>[2x]SQVRTYPNGLIVEELSMGKPNGKRADPGKTVSVRYIGKLQKNGKIFDSNIGKSPFKFRLGIGSVIKGWDVGVNGMR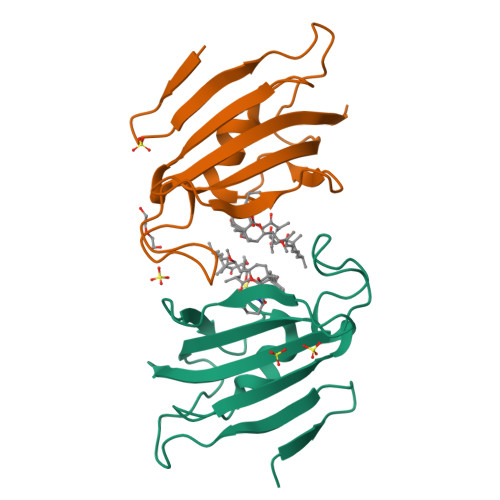VGDKRKLTIPPSMGYGVKGAGGQIPPNSWLTFDVELINVQLEHHHHHH N-(3,5-dimethoxyphenyl)imidodicarbonimidic diamide | C10 H15 N5 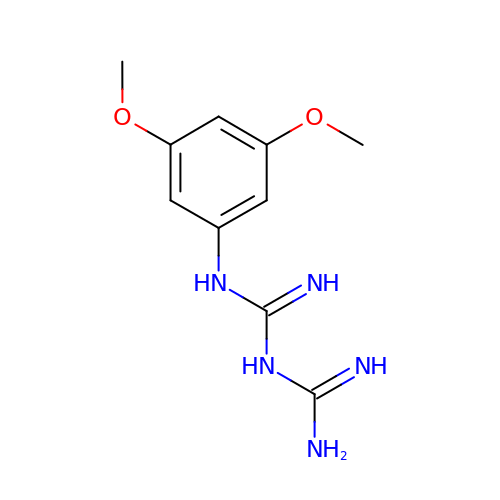O2 | VQKIGKHIRBCYNE-UHFFFAOYSA-N> NQPVNQPILAAAQSLHWEATKWSSKGNDIIAAAKRMALLMAEMSRLVRGGSGTKRALIQCAKDIAKASDEVTRLAKEVAKQC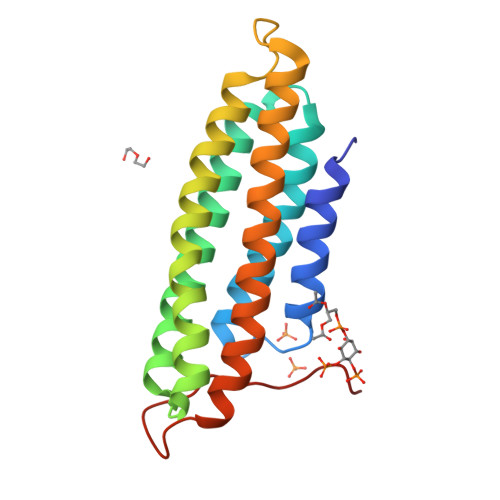TDKRIRTNLLQVCERIPTISTQLKILSTVKATMLGRTNISDEESEQATEMLVHNAQNLMQSVKETVREAEAASIKIRTDAGFTLRWVRKTPWYQ> SMIDDDGYRPNVGIVICNRQGQVMWARRFGQHSWQFPQGGINPGESAEQAMYRELFEEVGLSRKDVRILASTRNWLRYKLPKRLVRWDTKPVCIGQK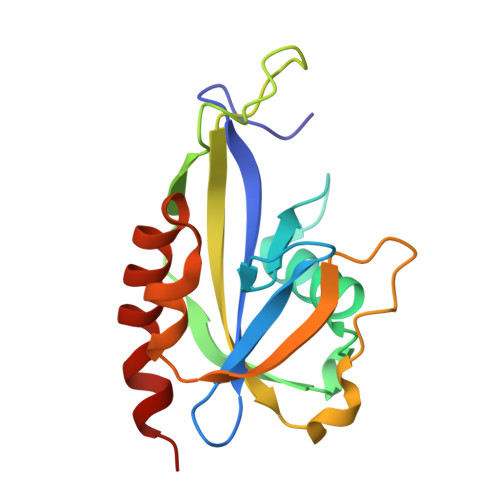QKWFLLQLVSGDAEINMQTSSTPEFDGWRWVSYWYPVRQVVSFKRDVYRRVMKEFASVVMSLAA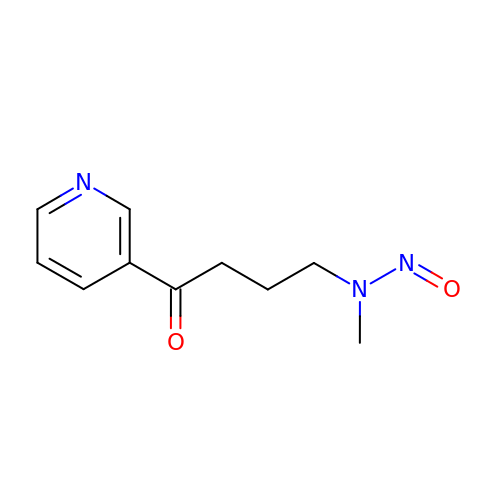4-[methyl(nitroso)amino]-1-(pyridin-3-yl)butan-1-one | C10 H13 N3 O2 | FLAQQSHRLBFIEZ-UHFFFAOYSA-N> GPGKT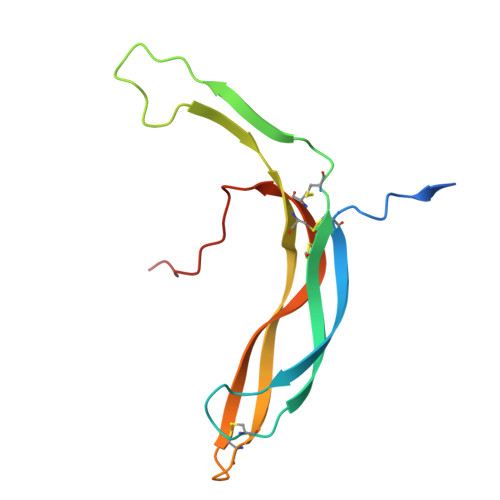DSSFIMDSDPRRCMRHHYVDSISHPLYKCSSKMVLLARCEGHCSQASRSEPLVSFSTVLKQPFRSSCHCCRPQTSKLKALRLRCSGGMRLTATYRYILSCHCEECNSGTETSQVAPA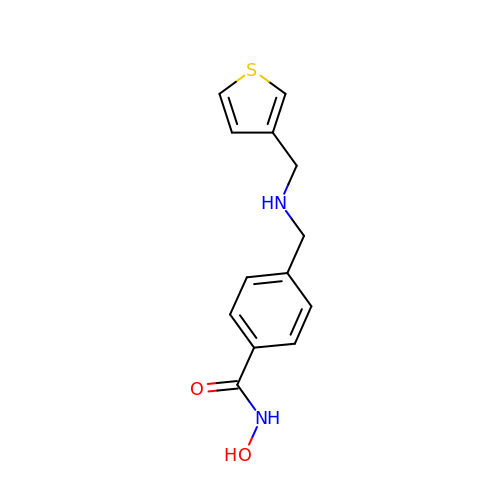N-hydroxy-4-({[(thiophen-3-yl)methyl]amino}methyl)benzamide | C13 H14 N2 O2 S | UUYNWXQYZUGELG-UHFFFAOYSA-N> KHLPEPFRIRVIEPVKRTTRAYREEAIIKSGMNPFLLDSEDVFIDLLTDSGTGAMTQSMQAAMMRGDEAYSGSRSYYALAESVKNIFGYQYTIPTHQGRGAEQIYIPVLIKKREQEKGLDRSKMVAFSNYFFDTTQGHSQINGCTVRNVYIKEAFDTGVRYDFKGNFDLEGLERGIEEVGPNNVPYIVATITSNSAGGQPVSLANLKAMYSIAKKYDIPVVMDSARFAENAYFIKQREAEYKDWTIEQITRETYKYADMLAMSAKKDAMVPMGGLLCMKDDSFFDVYTECRTLCVVQEGFPTYGGLEGGAMERLAVGLYDGMNLDWLAYRIAQVQYLVDGLEEIGVVCQQAGGHAAFVDAGKLLPH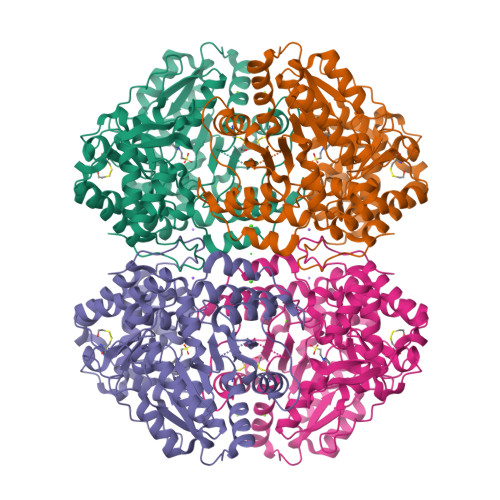IPADQFPAQALACELYKVAGIRAVEIGSFLLGRDPKTGKQLPCPAELLRLTIPRATYTQTHMDFIIEAFKHVKENAANIKGLTFTYEPKVLRHFTAKLKEV(1S,2R)-1-(4-hydroxy-3-methoxyphenyl)-2-(2-methoxyphenoxy)propane-1,3-diol 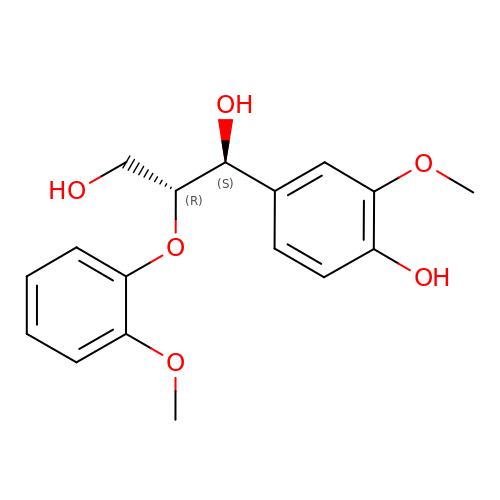| C17 H20 O6 | PPZSOILKWHVNNS-SJORKVTESA-N>GPLGSPNSQARPTVIRWSEGGKEVFISGSFNNWSTKIPLIKSHNDFVAILDLPEGEHQYKFFVDGQWVHDPSEPVVTSQLGTINNLIHVK[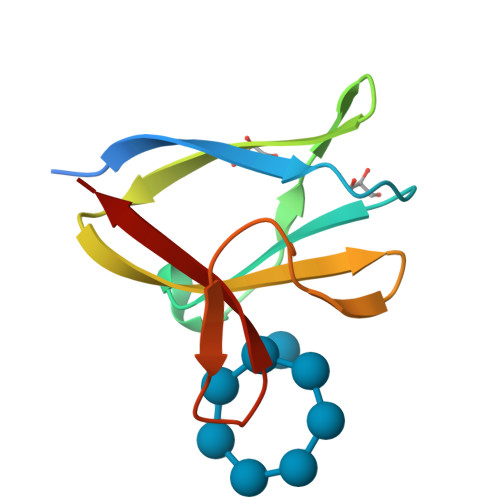18x]1-[2-(benzylamino)ethyl]-N-hydroxypiperidine-4-carboxamide | C15 H23 N3 O2 | 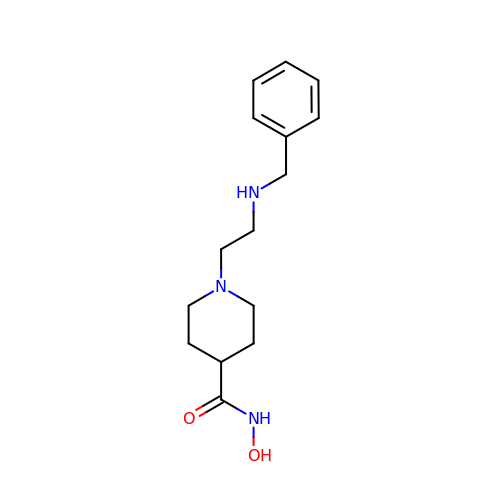IKRHDIZZKCLEPC-UHFFFAOYSA-N> NSVFSGLDMLILLPYERRGTRLVVEDYRPDHIYCIGADFGKNQDYSVFSVLDLD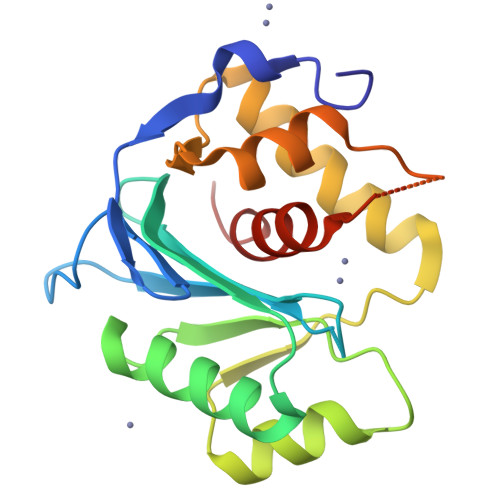TGAIACLERMNGATWSDQVARLKALSEDYGHAYVVADTWGVGDAIAEELDAQGINYTPLPVKSSSVKEQLISNLALLMEKGQVAVPNDKTILDELRNFRYYRTASGNQVMRAYGRGHDDIVMSLALAYSQYEG>MSAPTPLAEASQIPTIPALSPLTAKQSKGNFFSSNPISSFVVDTYKQLHSHRQSLELVNPGTVENLNKEVSRDVFLSQYFFTGLRADLNKAFSMNPAFQTSHTFSIGSQALPKYAFSALFANDNLFAQGNIDNDLSVSGRLNYGWDKKNISKVNLQISDGQPTMCQLEQDYQASDFSVNVKTLNPSFSEK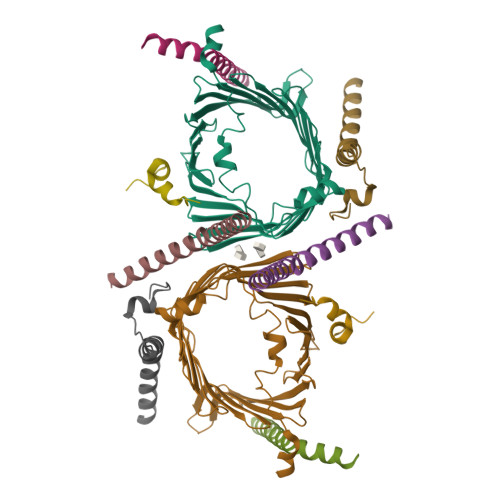GEFTGVAVASFLQSVTPQLALGLETLYSRTDGSAPGDAGVSYLTRYVSKKQDWIFSGQLQANGALIASLWRKVAQNVEAGIETTLQAGMVPITDPLMGTPIGIQPTVEGSTTIGAKYEYRQSVYRGTLDSNGKVACFLERKVLPTLSVLFCGEIDHFKNDTKIGCGLQFETAGNQELLMLQQGLDADGNPLQALPQLGGWSHPQFEK[2x];>[2x]MVELTEIKDDVVQLDEPQFSRNQAIVEEKASATNNDVVDDEDDSDSDFEDEFDENETLLDRIVALKDIVPPGKRQTISNFFGFTSSFVRNAFTKSGNLAWTLTTTALLLGVPLSLSILAEQQLIEMEKTFDLQSDANNILAQGEKDAAATANGGHHHHHHHH;>[2x]MFGLPQQEVSEEEKRAHQEQTEKTLKQAAYVAAFLWVSPMIWHLVKKQWK;>MDGMFAMPGAAAGAASPQQPKSRFQAFKESPLYTIALNGAFFVAGVAFIQSPLMDMLAPQL[2x];>[2x]MSFLPSFILSDESKERISKILTLTHNVAHYGWIPFVLYLGWAHTSNRPNFLNLLSPLPSV>SRHSEKIAIRDFQVGDLVLIILDERHDNYVLFTVSPTLYFLHSESLPALDLKPGEGASGASRRPWVLGKVMEKEYCQAKKAQNRFKVPLGTKFYRVKAVSWNKKV[2x];>[2x]SSGTSSEFEVVTPEEQ

Recent findings revealed that TNIP1 functions as a checkpoint mechanism that fine-tunes the rate of mitophagy by disrupting the recycling of the ULK complex during autophagosome formation. The phosphorylation of the TNIP1 FIR motif enhances its binding affinity for FIP200, enabling TNIP1 to compete with other autophagy receptors, such as CCPG1 or Optineurin. Here, we determined several crystal structures of the FIP200 claw domain in complex with phosphorylated TNIP1 FIR peptides and elucidated the specific recognition of different phosphorylated TNIP1 by FIP200 claw domain. Each FIP200 claw domain within the dimer features a five-stranded antiparallel β-sheet and a short α-helix.

The TNIP1 FIR_pS123 and p-CCPG1 FIR2 exhibited similar binding modes, but differences in C termini orientations could contribute to varying binding affinities to the FIP200 claw domain. To confirm this, we determined the complex structure of FIP200 claw domain with a novel peptide with an elongated C terminus (TNIP1_pS123long). The complex revealed that the elongated C-terminal residues of the new peptide were exposed to the solvent instead of interacting with β4 of the FIP200 claw domain. Then, 4-μs MD simulations for the FIP200–TNIP1_pS123long complex were conducted. FIP200 claw domain maintains stable throughout the entire simulation, with an RMSD of 2.6 Å. In contrast, the RMSD of TNIP1_pS123long peptide exhibits significant fluctuations between 1.2 and 6.0 Å, indicating its flexibility. To explore the origin of this flexibility, we calculated the RMSF of each Cα atom in the peptide. The analysis revealed that the central beta sheet of the peptide (F125-V127) is relatively stable, while the elongated tail of TNIP1_pS123long (T129-Q133) is quite flexible and disordered, consistent with experimental findings. In addition, according to further structural analysis and MD simulation, we revealed that the C-terminal elongated tail of TNIP1 peptide is flexible and affects the binding between FIP200 claw domain and TNIP1.>[4x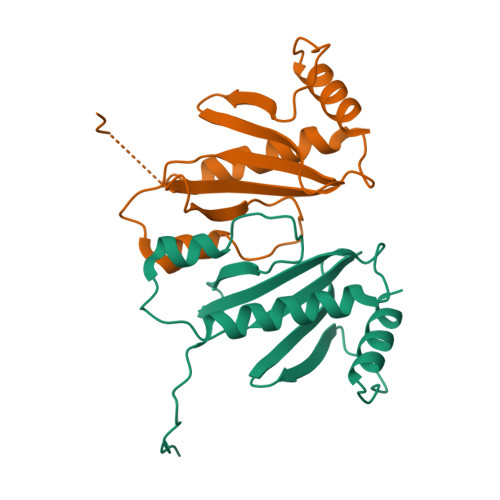]MYSFEQAITQLFQQLSLSIPDTIEPVIGVKVGEFACHITEHPVGQILMFTLPSLDNNNEKETLLSHNIFSQDILKPILSWDEVGGHPVLWNRQPLNNLDNNSLYTQLEMLVQGAERLQTSSLISPPRSFSPG>SQAAADRRTVEKTWKLMDKVVRLCQNPKLQLKNSPPYILDILPDTYQHLRLILSKYDDNQKLAQLSENEYFKIYIDSLMKKSKRAIRLFKEGKERMYEEQSQDRRNLTKLSLIFSHMLAEIKAIFPNGQFQGDNFRITKADAAEFWRKFFGDKTIVPWKVFRQC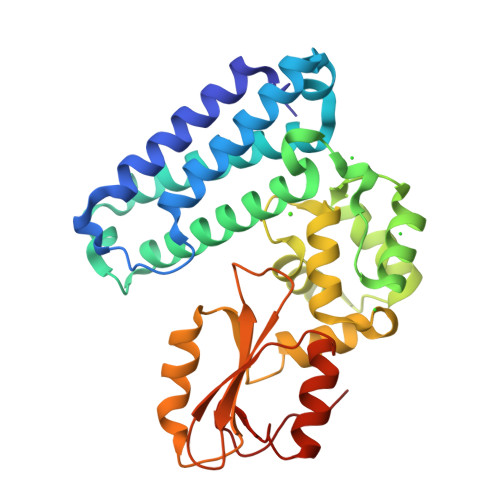LHEVHQISSGLEAMALKSTIDLTCNDYISVFEFDIFTRLFQPWGSILRNWNFLAVTHPGYMAFLTYDEVKARLQKYSTKPGSYIFRLSCTRLGQWAIGYVTGDGNILQTIPHNKPLFQALIDGSREGFYLYPDGRSYNPDLTG[3x];> DGYMP>[2x]MGSDSIDTPNYDVQKHINKLCGMLLITEDANHKFTGLIGM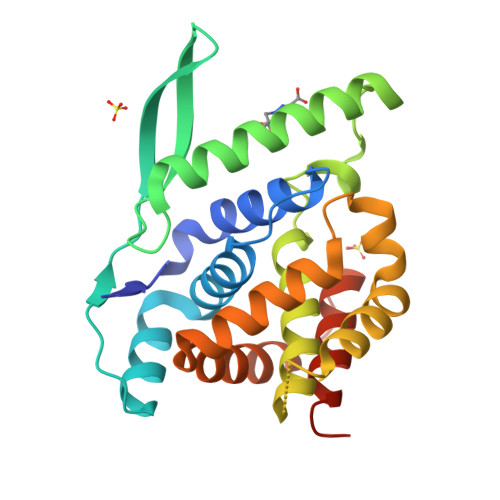LYAMSRLGREDTIKILRDAGYHVKANGVDVTTHRQDINGKEMKFEVLTLASLTTEIQINIEIESRKSYKKMLKEMGEVAPEYRHDSPDCGMIILCIAALVITKLAAGDRSGLTAVIRRANNVLKNEMKRYKGLLPKDIANSFYEVFEKHPHFIDVFVHFGIAQSSTRGGSRVEGIFAGLFMNAYGLEHHHHHH> MTQAEIKLCSLLLQEHFGEIVEKIGVHLIRTGSQPLRVIAHDTGTSLDQVKKALCVLVQHNLVSYQVHKRGVVEYEAQCSRVLRMLRYPRYIYTTKTLYSDTGELIVEELLLNGKLTMSAVVKKVADRLTETMEDGKTMDYAEVSNTFVRLADTHFVQRCPSVPTTENSDPGPPPPAPTLVINEKDMYLVPKLSLIGKGKRRRSSDEDAAGEPKAKRPKYTTDNKEPIPDDGIYWQANLDRFHQHFRDQAIVSAVANRMDQTSSEIVRTMLRMSEITTSSSAPFT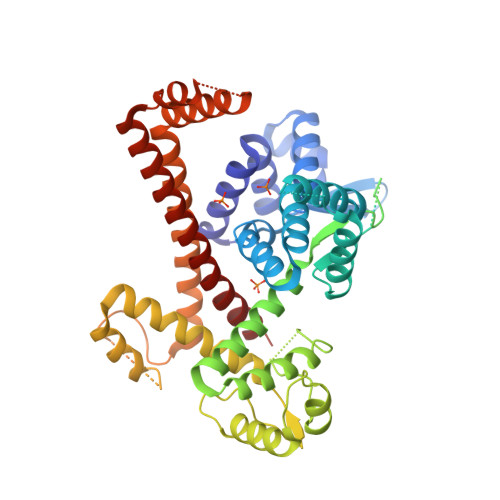QPLSSNEIFRSLPVGYNISKQVLDQYLTLLADDPLEFVGKSGDSGGGMYVINLHKALASLATATLESVVQERFGSRCARIFRLVLQKKHIEQKQVEDFAMIPAKEAKDMLYKMLSENFMSLQEIPKTPDHAPSRTFYLYTVNILSAARMLLHRCYKSIANLIERRQFETKENKRLLEKSQRVEAIIASMQATGAEEAQLQEIEEMITAPERQQLETLKRNVNKLDASEIQVDETIFLLESYIECTMKRQ4-({5-bromo-1'-[(2-chlorophenyl)sulfonyl]-2-oxospiro[indole-3,4'-piperidin]-1(2H)-yl}methyl)benzoic acid | C26 H22 Br Cl N2 O5 S | 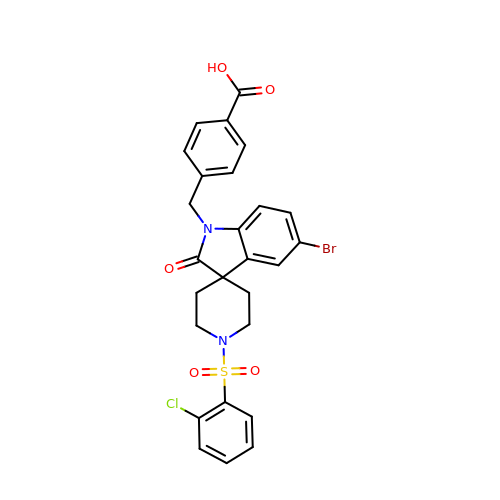SWIFZZMVSPDAPN-UHFFFAOYSA-N>SMANLRKVLISDSLDPCCRKILQDGGLQVVEKQNLSKEELIAELQDCEGLIVRSATKVTADVINAAEKLQVVGRAGTGVDNVDLEAATRKGILVMNTPNGNSLSAAELTCGMIMCLARQIPQATASMKDGKWERKKFMGTELNGKTLGILGLGRIGREVATRMQSFGMKTIGYDPIISPEVSASFGVQQLPLEEIWPLCDFITVHTPLLPSTTGLLNDNTFAQCKKGVRVVNCARGGIVDEGALLRALQSGQCAGA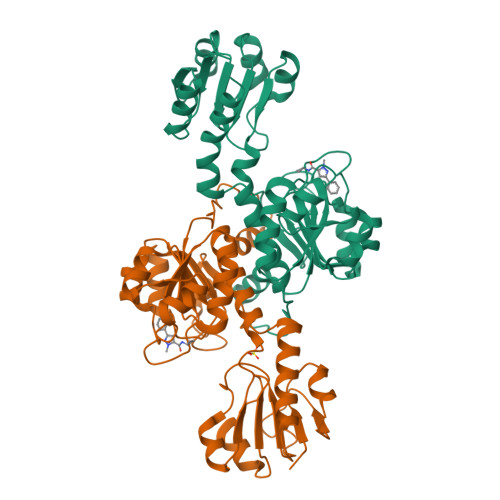ALDVFTEEPPRDRALVDHENVISCPHLGASTKEAQSRCGEEIAVQFVDMVKGKSLTGV[2x]> MGSSHHHHHHSQDPMDYFNIKQNYYTGNFVQCLQEIEKFSKVTDNTLLFYKAKTLLALGQYQSQDPTSKLGKVLDLYVQFLDTKNI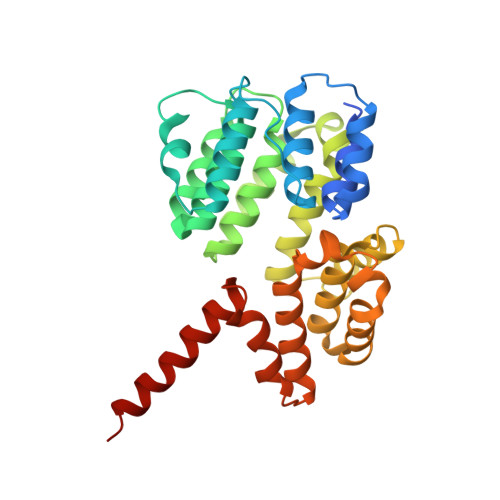EELENLLKDKQNSPYELYLLATAQAILGDLDKSLETCVEGIDNDEAEGTTELLLLAIEVALLNNNVSTASTIFDNYTNAIEDTVSGDNEMILNLAESYIKFATNKETATSNFYYYEELSQTFPTWKTQLGLLNLHLQQRNIAEAQGIVELLLSDYYSVEQKENAVLYKPTFLANQITLALMQGLDTEDLTNQLVKLDHEHAFIKHHQEIDAKFDELVRKYDTSN> MKHHHHHHSAGLEVLFQGPMEDGEVNDVVHPQVRAHINSLVSALGGISIDDDGGYKLGDDALEVLRDLKKWIRFYDEKTNRMDVARCLAEANIVSTDLLHILALWTPNENSNKYKARIALACFELMVPLTWPIEKDRETMTINHHRHIPVLQLAQLGYKRAIINYDAAPILSTAVRVALPAMAMPIGERTARDQGIIKLILYFLRNIAMITPPPGVKYEGDESQISRSALIDAFSYQDIFLTLLTIASNMGEDFRTEDVIVMEIIFHLVKRVDPKGQQLGSFVSDFLDSGFNPLFSHIRKSLEREAPHVLHYHQSQFFYLVAWFLEAERARRSSFNLIASVLTQ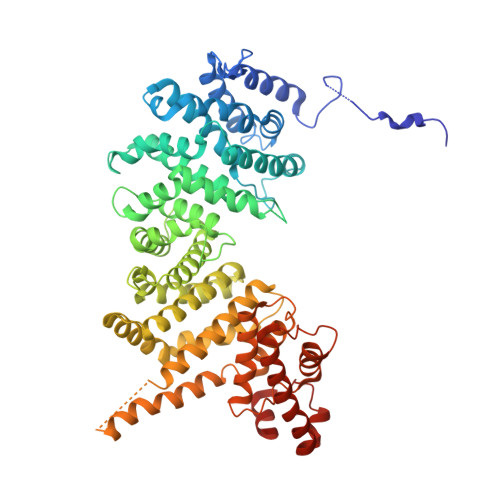EMFIALNRALDRAYGDKDWRLLTSAMRCFTQILLTVQEMFDSGNDEDQEIADNILSRLFYEESTHDAVANIVRTYKDQGFEYLDACTELAHTFLRILEAYSKQNVDLQVRSGSADDEKMAEKTSQERKFDFKRFAARFTPQGVVDTFVTFTKYYRDLDDSQLKRAHRYFYRVAFKQEMSVMLFRLDIIHLFYNMIKGPEPLDKNSPMYKEWEELVRQILKRCIRKLEERPALFTEILFSKINSTAYYLEYGFEKQ N-hydroxy-5-sulfanylpentanamide | C5 H11 N O2 S | 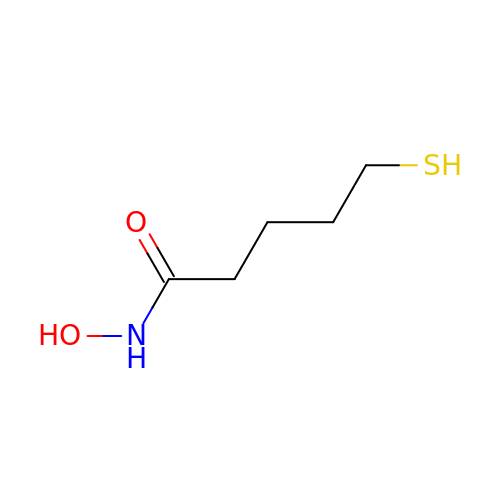FTZSDBLOZDZSRD-UHFFFAOYSA-N Although most signal via cyclic oligoadenylate, an alternative class of signalling molecule SAM-AMP, formed by conjugating ATP and S-adenosylmethionine, was described recently. SAM-AMP activates a trans-membrane effector of the CorA magnesium transporter family to provide anti-phage defence. NrN is replaced by a SAM-AMP lyase in some CorA-associated type III CRISPR systems, including that from Clostridium botulinum. SAM-AMP lyase exhibits a typical trimeric PII-like protein architecture characterized by a triangular core formed by the four-stranded antiparallel β-sheet of each subunit.

Purified WT SAM-AMP lyase was crystallized, X-ray data were collected to 1.70 Å resolution, and the structure was solved using molecular replacement. The asymmetric unit contains six copies of SAM-AMP lyase, with two trimeric complexes. Each monomer possesses a signature ferredoxin fold (β1-α1-β2-β3-α2-β4), featuring a β-sheet on one side and two α-helices on the other. The β2 and β4 strands from each of the three subunits interact in a ‘head-to-tail’ orientation, contributing to most of the trimeric interface. The T-loop connecting β2 and β3, which plays a key role in interactions with target proteins in canonical PII proteins, is shorter (10–12 residues in SAM-AMP lyase/SAM lyase compared to >20 residues in homologues) and presumably less flexible in SAM-AMP lyase/SAM lyase (given the loops are fully modelled in the lyases, but missing in the homologues, despite similar data resolution). Comparison of the apo SAM-AMP lyase and in complex with MTA-AMP reveals almost identical structures (root mean square deviation (RMSD) of 0.3 Å over 123 Cα atoms), consistent with the slight conformational change observed in the homologous SAM-lyase (Svi3-3) upon SAM binding. This suggests the proteins essentially have a pre-formed binding site for ligands. Given the proximity of the T-loop to the binding site of MTA-AMP, it is perhaps surprising that there is no significant movement of this upon binding. However, the side chain of W64, which could only be modelled in some monomers suggesting that it is highly flexible, appears to move through 90° from a position that would clash with SAM-AMP to a conformation promoting the π-stacking interaction with the adenine base of the AMP. This residue may serve as a gatekeeper to the binding site, locking the SAM-AMP substrate in position for catalysis.

>[6x]GANAMAHMGKTLRFEIVSGVNKGYFHTNSQSESLDLVGGIWQKIAKEEFEKSNIYVSAVIKPSKTVYNQEWGCPENGEETVVLTGVANEEFVDDIEKWKDTVIKLAKELKNQMKQSTLTCEFIETELHYFK> SAADVFVPDEWEVAREKITMSRELGQGSFGMVYEGVAKGVVKDEPETRVAIKTVNEAASMRERIEFLNEASVMKEFNCHHVVRLLGVVSQGQPTLVIMELMTRGDLKSYLRSLRPEMENNPVLAPPSLSKMIQMAGEIADGMAYLNANK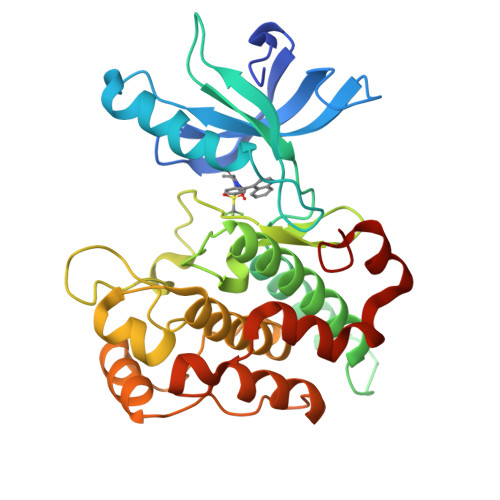FVHRDLAARNCMVAEDFTVKIGDFGMTRDIYETDYYRKGGKGLLPVRWMSPESLKDGVFTTYSDVWSFGVVLWEIATLAEQPYQGLSNEQVLRFVMEGGLLDKPDNCPDMLFELMRMCWQYNPKMRPSFLEIISSIKEEMEPGFREVSFYYSEENK> MRRGIVNHYYWSRYRMPTQMPKFDGPAPIAAPQNMNSTKTNEFIDPIDDKFPLSIRGPLVRPDVPEDQYVDSWYVCTSMTHHLGDYRPWSASAPPNAYRFRPYNEFDAKGREYVEYMRQFARYDPRKSQGKGQKGFPFRDAYLTKMNEANRTTPPPTLETIMDRAVREKHQHARVLSPMQVQRDVGRSETPLPCAGNIPVDRSQFPFCWKTEDWYEYEVAKVRNKRFVFENTEEDGIHGSEVTYKIVLEGFWDHHVMKLAEDVCMFLRDVGRQVTEEKLVAVRRVMEGLTGGAFDPELIDFFNAARAGPFGRPDEYDAEEVANFVRADLKRLEEQCLNVINRCNVPVPGATNIYDPQVSWPYVEKLEPWVRMAEFWTSSSDTSFTELEMSTAHYEFRKYFRVIICKLPFQSTEFEKRMYDIRHWLHRQTTCEFHTIYRKNVIHDGSVFPTEHDPATPTTHDHHRMFSFALDWQSAPVNRLSVARVLEGDDWERVAQRLGCSVDDLKEANPAIEEL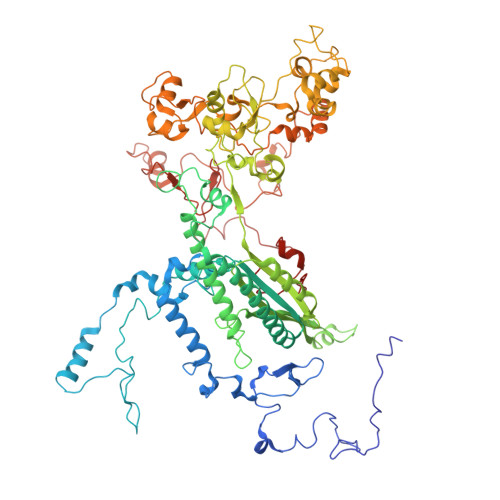EAGAVLNVPGGASRRLTSFGAAPRVLPLQNPNNGKRIRTWEDAATVLDCTVEELQQANGHAALTYKQTGENGEGEFGPSVTELNVPLSCWVSTAETEFSPVELVFAGDTFATIAQRLRCSEEALKKANDGQSDLSHARFVRVPAEAKAPRRLLEPQLRSQAATDVLMTRTIAEEAAYGIKNIPDLPSNASKFPHEYHTPTSRFPTTPKEKESESDWMAYTARYLDKQFTHPTEPTPIYNVNKLWPMQQVPGKIDQTPFEEDQTWLLNPIPVQQLEQHHPEKDLQDLPFVNHEQFPRSLEWTAP> 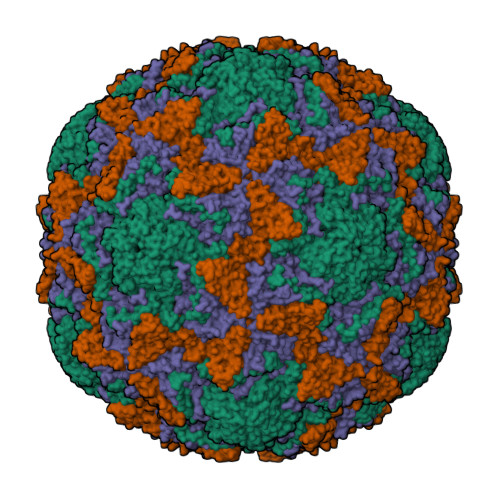GDNQDRTVANTQPSGPSNSTEIPALTAVETGHTSQVDPSDTIQTRHVVNFHSRSESTIENFMGRAACVFMDQYKINGEETSTDRFAVWTINIREMAQLRRKCEMFTYMRFDIEMTMVITSCQDQGTILDQDMPVLTHQIMYVPPGGPIPAKVDGYEWQTSTNPSVFWTEGNAPPRISIPFISVGNAYSSFYDGWSHFTQDGTYGYTTLNAMGKLYIRHVNRSSPHQITSTIRVYFKPKHIKAWVPRPPRLCPYINKRDVNFVVTEITDSRTSITDTPHPEHSVLATH;> SPSAEECGYSDRVRSMTLGNSTITTQESANVVVGYGEWPSYLSDREATAEDQPTQPDVATCRFYTLESVQWEKTSPGWWWKFPEALKNMGLFGQNMHYHYLGRAGYTIHVQCNASKFHQGCLLVVCVPEAEMGCADTDTTFPATELTTEDTPHVFTSDSITGKKVQAAVCNAGMGVGVGNLTIFPHQWINLRTNNSATIVIPYINSVPMDNMFRHYNFTLMIIPFAPLNFTDGATAYVPITVTIAPMYAEYNGLRLASTQ;> GVPVLNTPGSNQFLTSDDYQSPSAMPQFDETPEMHIPGEVRNLMEIAEVDSVVPVNNVTGKTKSMDAYQIPVGTGNTDKTKPIFSFQMDPGYSSVLKRTLLGEMLNYYAHWSGSVKLTFLFCGSAMATGKLLISYSPPGASVPTSRKDAMLGTHIVWDIGLQSSCVLCVPWISQSHYRMVQQDPYTSAGYITCWYQTNIVVPPGAPTSCDVLCFASACNDFSVRLLRDTPFMAQPGKLQ;> MGAQVSTQKTGAHETSLSAKGNSIIHYTNINFYKDAASSASNRQDIQQDPGKFTDPVKDLMIKTLPALN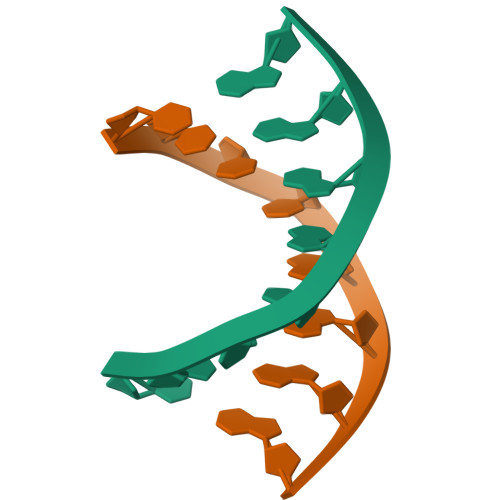> CTCTAGAG> HMSLSVANSTYETTALNSQKSSTDQPNSGSKSGQTL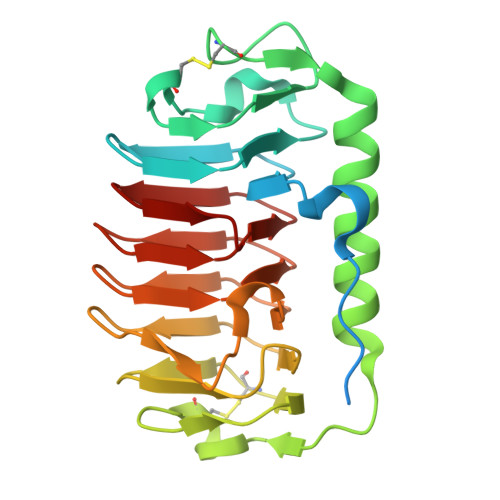DLVNLGVAANFAILSKTGITDVYKSAITGDVGASPITGAAILLKCDEVTGTIFSVDAAGPACKITDASRLTTAVGDMQIAYDNAAGRLNPDFLNLGACTIGGKTLTPGLYKWTCTLNIPTDITISGSSTDVWIFQVAGNLNMSSAVRITLAGGAQAKNIFWQTAGAVTLGSTSHFEGNILSQTGINMKTAASINGRMMAQTAVTLQMNTVTIPQ>[11x]MELIHPENGPSGTVQVPLIQGVDQSDTEDVYRLSPHVTTGFADTFKESNDIMGFSFMEKVNGAIYKYTHFAFYAVLNLLLAPFIAFSFGLSFAVMHFAVVWFVQPIMKLYYVWLRVFNLAYEPALRLVCDPIHRSIALILSGIKGQFKMNSSDVKTSQV

Caveolins are a unique family of membrane remodeling proteins present broadly across animals (Metazoa), and in vertebrates form flask-shaped invaginations known as caveolae. Unlike vesicle coat proteins such as clathrin, COPI, and COPII that cycle on and off membranes and share evolutionary origins and structural features, caveolins are unrelated in sequence to other vesicle coat proteins and remain integrated in membranes throughout their life cycle. Using a combination of computational and structural approaches, we now show that caveolins across evolution share the ability to assemble into amphipathic disk–shaped multimers composed of spiraling α-helices and a central protruding parallel β-barrel. Each complex forms a disk with 11 spiraling α-helices and a central β-barrel, with each protomer forming contacts with two protomers to the left and two to the right.

We used single-particle cryo-EM to determine a 3.1 Å resolution structure of the S. purpuratus caveolin complex and built a model spanning amino acids 29–152. Residues 1–28 and 153–159, regions predicted to be disordered, were not visible in the map. The complex, ∼130 Å in diameter and ∼36 Å in height, is composed of 11 spiraling α-helical protomers organized into a disk with a protruding β-barrel. The variable N-terminal region extends along the cytoplasmic face of the complex before making a 180° turn at the hook structure. Amphipathic α-helices form the spoke region, with the α-1 helix forming the rim of the disk that is ∼15 Å in height, and the C terminus of each protomer is a β-strand that forms a central parallel β-barrel ∼30 Å in diameter. An unstructured detergent micelle covers the hydrophobic face of the disk and reaches into the interior of the β-barrel, suggesting both regions interact with membrane. Comparison of the experimental and AF2.2 structures shows the computational model did not correctly predict the length of the β-barrel or the curvature of the disk. 2D averages of vitrified S. purpuratus caveolin complexes showed variations of curvature, including examples of complexes with either concave or convex curvatures. Calculated using a filter resolution of 8 Å, these low-resolution structures represent the negative and positive values along the reaction coordinate for the component with the largest variance. This analysis shows that the S. purpuratus caveolin disk can be concave, similar to the 3.1 Å structure, or can be flat. Thus, we conclude that the S. purpuratus caveolin complex is more flexible than the human or S. rosetta caveolin complexes under these experimental conditions.>MLEADDQGCIEEQGVEDSANEDSVDAKPDRSSFVPSLFSKKKKNVTMRSIKTTRDRVPTYQYNMNFEKLGKCIIINNKNFDKVTGMGVRNGTDKDAEALFKCFRSLGFDVIVYNDCSCAKMQDLLKKASEEDHTNAACFACILLSHGEENVIYGKDGVTPIKDLTAHFRGDRCKTLLEKPKLFFIQACRGTELDDGIQADSGPINDTDANPRYKIPVEADFLFAYSTVPGYYSWRSPGRGSWFVQALCSILEEHGKDLEIMQILTRVNDRVARHFESQSDDPHF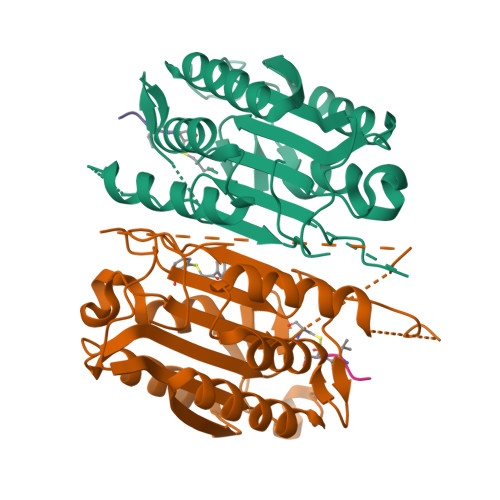HEKKQIPCVVSMLTKELYFSQ[2x]>SNAVIRPKTLGQKHYVDAIDTNTIVFGLGPAGSGKTYLAMAKAVQALQSKQVSRIILTRPAVEAGEKLGFLPGTLNEKIDPYLRPLHDALRDMVEPEVIPKLMEAGIVEVAPLAYMRGRTLNDAFVILDEAQNTTPAQMKMFLTRLGFGSKMVVTGDITQVDLPGGQKSGLRLVRHILRGVDDVHFSELTSSDVVRHQLVGHIVD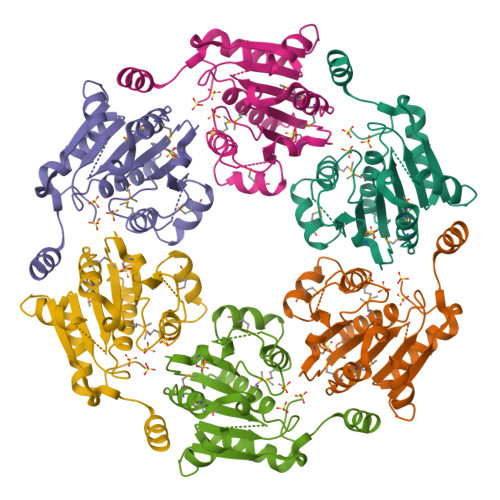AYE[2x]>MAPVKVFGPAMSTNVARVTLCLEEVGAEYEVVNIDFNTMEHKSPEHLARNPFGQIPAFQDGDLLLWESRAISKYVLRKYKTDEVDLLRESNLEEAAMVDVWTEVDAHTYNPALSPIVYQCLFNPMMRGLPTDEKVVAESLEKLKKVLEVYEARLSKHSYLAGDFVSFADLNHFPYTFYFMATPHAALFDSYPHVKAWWDRLMARPAVKKIAATMVPPKA[6x]

In black-grass, upregulation of a phi (F)-class GST1 (AmGSTF1) has been shown to be a functional biomarker of MHR. Recombinant AmGSTF1 has been shown to exhibit both glutathione-S-transferase activity toward xenobiotics, as well as acting as a GPOX, reducing fatty-acid hydroperoxides to less reactive monohydroxy derivatives. The Phi (F) class GSTs, of which AmGSTF1 is an example, are found in all higher plants, being homodimeric enzymes in which each protomer of approximately 23–30 kDa with the catalytic serine residues located at the interface. Each protomer has two distinct domains; the N-terminal domain adopts the typical thioredoxin-fold, with the C-terminal domain being a bundle of at least five helices as demonstrated by the crystal structures of AmGSTF1 presented here.

To explore how AmGSTF1 can be regulated by chemical inhibitors, a series of crystal structures of the native protein was determined. The first two crystal modifications obtained, hexagonal and rhombohedral, diffracted to 1.53 Å and 1.95 Å resolution, respectively (Table S1a‡). The hexagonal modification contained one protein chain in the asymmetric unit, whereas the rhombohedral form had six independent molecules with a very similar packing arrangement of trimers composed of the functional GST dimer. All polypeptide chains adopted virtually identical overall structures, with rmsds ranging from 0.2–0.4 Å on Cα-atoms. In both crystal modifications, the four residues preceding this loop, (Cys120-Leu121-Phe122-Asn123), were found to project into the monomer subunit of a symmetry-related chain, effectively blocking the active site of the adjacent subunit. This arrangement explains why no ligands were found to be bound in either the G- or the H-site of this open-loop apo-structure, with both loops being flexible and presumably closing upon ligand binding.> SMNIQALLSEKVRQAMIAAGAPADCEPQVRQSAKVQFGDYQANGMMAVAKKLGMAPRQLAEQVLTHLDLNGIASKVEIAGPGFINIFLDPAFLAEHVQQALASDRLGVATPEKQTIVVDYSAPNVAKEMHVGHLRSTIIGDAAVRTLEFLGHKVIRANHVGDWGTQFGMLIAWLEKQQQENAGEMELADLEGFYRDAKKHYDEDEEFAERARNYVVKLQSGDEYFREMWRKLVDITMTQNQITYDRLNVTLTRDDVMGESLYNPMLPGIVADLKAKGLAVESEGATVVFLDEFKNKEGEPMGVIIQKKDGGYLYTTTDIACAKYRYETLHADRVLYYIDSRQHQHLMQAWAIVRKAGYVPESVPLEHHMFGMMLGKDGKPFKTRAGGTVKLADLLDEALERARRLVAEKNPDMPADELEKLANAVGIGAVKYADLSKNRTTDYIFDWDNMLAFEGNTAPYMQYAYTRVLSVFRKAEIDEEQLAAAPVIIREDREAQLAARLLQFEETLTVVAREGTPHVMCAYLYDLAGLFSGFYEHCPILSAENEEVRNSRLKLAQLTAKTLKLGLDTLGIETVERM

The arginyl-tRNA synthetase (ArgRS) catalyzes the esterification reaction between L-arginine and its cognate tRNAArg. A member of the class I aaRS, the arginyl-tRNA synthetase (ArgRS) possesses several distinct characteristics. To better recognize these identity elements, ArgRS possesses an N-terminal domain of roughly 100 amino acids—the Add1 domain, which is unique among aaRSs. Here we report the first crystal structure of E. coli ArgRS (eArgRS) complexed with L-arginine, and a series of mutational studies using isothermal titration calorimetry (ITC).

E. coli ArgRS contains the N-terminal additional domain (Add1, residues 1–112), the catalytic domain (113–382) including two insertion domains (Ins1, residues 164–221, and Ins2, residues 258–311), and the C-terminal additional domain (Add2, 383–577). The refined structure contains the whole sequence except residues Q178–A187, D203–E204 and the C-terminal M577. The crystallographically invisible residues (178–187 and 203–204) are part of the insertion domain 1 (Ins1) as defined by Cavarelli and co-workers. A well-ordered L-arginine binds in the active site of the catalytic domain. Although 2.5 mmol/L ATP was always present in the crystal growth solution, ATP molecule is not visible in the electronic density map. Three residues in the region (A121, N123 and H132) formed hydrogen bonds to the main chain atoms of L-arginine and adopted similar orientations as observed in yeast structures (Asn153 and Gln375 of yArgRS), independent of tRNA binding. The side chain recognition motif, which dictates the specificity of the enzyme, contains three conserved residues (D118, Y313, D317) making direct H-bonds (or salt bridges) to the guanidinium moiety of arginine. Another residue R324 formed two hydrogen bonds with D118, stabilizing the orientation of the latter. A closer look at the active site of the eArgRS-L-arginine complex revealed a closed loop of hydrogen bonding moieties, consisting of L-arginine, Q341 and Y313. In particular, Y313 of eArgRS acts as a gate-keeper: keeping the binding pocket open in the absence of arginine via the Y313-W162 H-bond, while locking the bound arginine in position after rotameric rotation.SA lipase (SAL, also known as glycerol ester hydrolase), a triacylglycerol esterase, shows strong cytopathic activity in host cells. SAL, an ester bond-hydrolyzing enzyme, is secreted in prepolypeptide form containing 690 amino acid residues and is processed into its mature form containing 394 amino acid residues. Its active site is composed of a typical catalytic triad including Ser116, Asp 307, and His349 residues, similar to other serine hydrolases. The SAL crystal structure exhibited a typical α/β-hydrolase fold comprising a central twisted β-sheet flanked by α-helices on both sides.

We screened various chemical libraries and discovered that the anti-obesity drug orlistat is a potent SAL inhibitor with an IC50 value of 2.4 μM. The crystal structure of the SAL–orlistat complex showed an inhibitor-binding site and atomic-level details of binding interactions. Notably, the β-lactone rings of orlistat molecules were decyclized by their hydrolyzing ring cleavage reaction with SAL on chains A and B. Ser116 attached the carbonyl carbon atom of the orlistat tetracyclic rings at the active sites. Then, orlistat covalently bound to Ser116, with the oxygen atom of Ser116 and orlistat maintaining the bond. SAL monomer bound one orlistat molecule each in a similar manner. The oxygen atom of the hydroxy group is hydrogen bound to the His349 side-chain nitrogen atom (2.67 Å). The Ser116 side-chain residue covalently bound to the carboxylate group and shared one oxygen atom with both SAL and orlistat. The other oxygen of the decycled carboxylate group formed hydrogen bonds with two nitrogen atoms of the main chain Phe17 (2.97 Å) and Met117 (2.75 Å), which form the oxyanion hole. The terminal N-formyl carbonyl group of the amino ester moiety was located in the hydrophobic pocket formed by Leu18, Tyr29, Pro30, Tyr32, Val350, Ile353, and Val355. The α-side chain of orlistat was also primarily bound to a hydrophobic pocket, which was formed by Ala174, Ala176, Pro168, Leu242, Val309, Val310, and partially Phe17 at the bottom of its deep active site. The SAL–orlistat complex also had an open form, with the lid region located as far as possible from the catalytic cavity.

>MNHKVHHHHHHMKANQVQPLNKYPVVFVHGFLGLVGDNAPALYPNYWGGNKFKVIEELRKQGYNVHQASVSAFGSNYDRAVQLYYYIKGGRVDYGAAHAAKYGHERYGKTYKGIMPNWEPGKKVHLVGHSMGGQTIRLMEEFLRNGNKEEIAYHQAHGGEISPLFTGGHNNMVASITTLATPHNGSQAADKFGNTEAVRKIMFALNRFMGNKYSNIDLGLTQWGFKQLPNESYIDYIKRVSKSKIWTSDDNAAYDLTLDGSAKLNNMTSMNPNITYTTYTGVSSHTGPLGYENPDLGTFFLMDTTSRIIGHDAREEWRKNDGVVPVISSLHPSNQPFVNVTNNEPATRRGIWQVKPILQGWDHVDFIGVDFLDFKRKGSELANFYIGIINDLLSVEATEGKGTQLKAS[2x]The kinase RIP1, acting downstream of TNFR1 (tumor necrosis factor receptor 1), can trigger apoptosis through binding to FADD, the activating adaptor for caspase-8, or necroptosis through binding to RIP3. Although the kinase activity of RIP1 is dispensable for NF-κB and MAPK signaling by TNFR1, it is essential for interactions between RIP1 and RIP3 that activate RIP3 to phosphorylate MLKL. The kinase activity of RIP1 has been implicated in many pathologies characterized by inflammation and tissue damage. The kinase domain of RIP1 has unique structural features, which allow the development of selective RIP1 inhibitors.

To investigate the potential therapeutic benefit of inhibiting RIP1, we developed GNE684 or (S)-N-((S)-7-methoxy-1-methyl-2-oxo-2,3,4,5-tetrahydro-1H-pyrido[3,4-b]azepin-3-yl)-5-phenyl-6,7-dihydro-5H-pyrrolo[1,2-b][1,2,4]triazole-2-carboxamide with cross-species potency against RIP1, exquisite kinase selectivity, and favorable pharmacological properties. A co-crystal structure showed that GNE684 binds to the same hydrophobic pocket within the kinase domain of RIP1 that is bound by necrostatins. GNE684 binds to an inactive conformation of RIP1, similar to type II kinase inhibitors, with the Asp156 and Leu157 of the DLG motif (commonly DFG in other kinases) in the “out” conformation and the αC helix swung away from the ATP-binding cleft, and lacking the canonical ion pair between the catalytic lysine (Lys45) and αC glutamate (Glu63). GNE684 inhibited human RIP1 potently in vitro, and mouse and rat RIP1 with slightly less potency. Accordingly, it inhibited TNF-induced necroptosis in human HT-29, mouse L929, or rat H9c2 cells. Accordingly, GNE684 disrupted TBZ-induced RIP1 autophosphorylation, interactions between RIP1 and RIP3, RIP3 autophosphorylation, and phosphorylation of MLKL by RIP3. Consistent with observations in cells expressing kinase-dead RIP1 mutant D138N, GNE684 did not affect RIP1 protein abundance or TNF-induced activation of NF-κB or MAPK (JNK) signaling, even at elevated concentrations (20 and 200 μM). However, interspecies differences in RIP1 mean that inhibitors blocking human RIP1 can be over a hundred-fold weaker against murine RIP1. Although slightly more potent against human RIP1, GNE684 can also inhibit mouse RIP1 effectively. GNE684 provided much the same level of protection as genetic inactivation of RIP1 in several inflammatory disease models (TNF-driven SIRS, colitis induced by NEMO deficiency in IECs, and collagen antibody-induced arthritis).

>GSMQPDMSLNVIKMKSSDFLESAELDSGGFGKVSLAFHRTQGLMIMKTVYKGPNCIEHNEALLEEAKMMNRLRHSRVVKLLGVIIEEGKYSLVMEYMEKGNLMHVLKAEMSTPLSVKGRIILEIIEGMAYLHGKGVIHKDLKPENILVDNDFHIKIADLGLASFKMWSKLNNEEHNELREVDGTAKKNGGTLYYMAPEHLNDVNAKPTEKSDVYSFAVVLWAIFANKEPYENAIAEQQLIMAIKSGNRPDVDDITEYCPREIISLMKLCWEANPEARPTFPGIEEKFRPFYLSQLE[2x]>MVVSIGVFDGVHIGHQKVLRTMKEIAFFRKDDSLIYTISYPPEYFLPD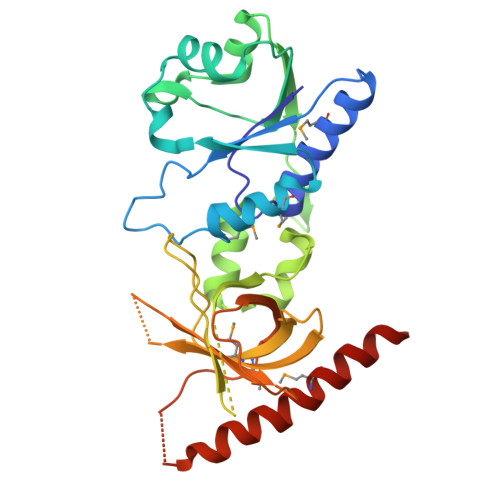FPGLLMTVESRVEMLSRYARTVVLDFFRIKDLTPEGFVERYLSGVSAVVVGRDFRFGKNASGNASFLRKKGVEVYEIEDVVVQGKRVSSSLIRNLVQEGRVEEIPAYLGRYFEIEGIVHKDREFGRKLGFPTANIDRGNEKLVDLKRGVYLVRVHLPDGKKKFGVMNVGFRPTVGDARNVKYEVYILDFEGDLYGQRLKLEVLKFMRDEKKFDSIEELKAAIDQDVKSARNMIDDIINSKFEKEG[2x]> QAISEKDRGNGFFKEGKYERAIECYTRGIAADGANALLPANRAMAYLKIQKYEEAEKDCTQAILLDGSYSKAFARR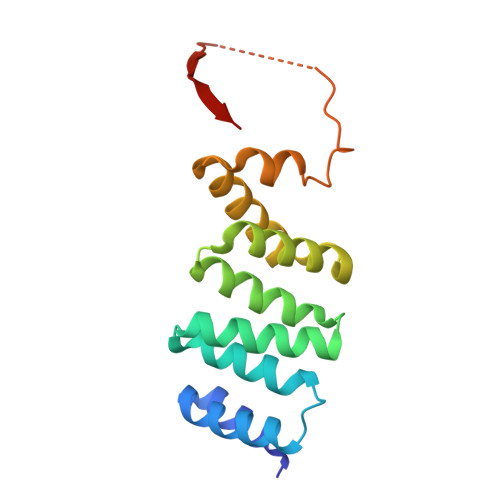GTARTFLGKLNEAKQDFETVLLLEPGNKQAVTELSKIKKELIEKGHWDDVFLDSTQRQNVVKPIDNPPHPGSTKPLKKVIIEETGNLIQ> MELPRAFGLLLHPTSLPGPYGVGVLGQEARDFLRFLKEAGGQYWQVLPLGPTGYGDSPYQSFSAFAGNPYLVDLRPLAKRGYVRLEDPGFPQGRVDYGLLYAWKWPALKEAFRGFQEKAPPEEREDFAAFREKEAWWLEDYALFMALKGAHGGLPWNRWPLPLRKREEQALREAKSALAEEVAFHAFTQWLFFRQWGALKAEAEALGIRILGDMPIFVAEDSAEVWAHPEWFHLDEEGRPTVVAGVPPDYFSETGQRWGNPLYRWDVLEREGFSFWIRRLEKALELFHLVRIDHFRGFEAYWEIPASCPTAVEGRWVKAPGEKLFQKIQETFGQVPILAEDLGVITPEVEALRDRFGLPGMKVLQFAFDDGMENPFLPHNYPSHGRVVVYTGTHDNDTTLGWYRTATPHEKAFMARYLADWGIFFREEEEVPWALMRLGMKSVARLAVYPVQDVLALGSEARMNYPGRPSGNWAWRLLPGELSPEHG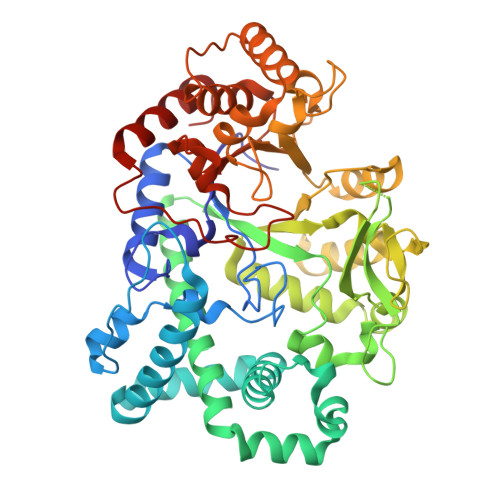ERLRAMAEATERL>MFRIGQGFDVHQLVEGRPLIIGGIEIPYEKGLLGHSDADVLLHTVADACLGAVGEGDIGKHFPDTDPEFKDADSFKLLQHVWGIVKQKGYVLGNIDCTIIAQKPKMLPYIEDMRKRIAEGLEADVSQVNV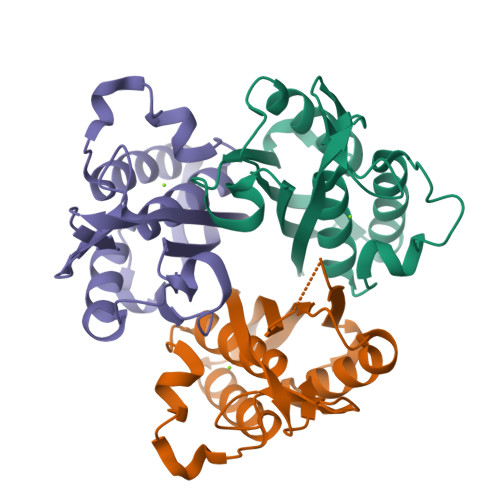KATTTEKLGFTGRAEGIAAQATVLIQKG[6x]> MANVNKVVRRRQVALLIALVLGIGAGGAGTWMVSEMNLKKAPPAKAPKGEPAPDMTGVVNQSFDNKVQRSAIAEAQRLNKETQTEIKKLRTEMGLVSRDLKGSQDRIRELEDQNQLLQTQLEAGKNFDSLSAEPLPGALASQGKPAPAGNVPPPTSFWPAGGGQAPAAPVMTPIQRPGMMDSQEFSLPDTGPKKPRFPWISSGSFVEAIVVEGADANASVTGDKNTAPMQLRLTGKVQMPNDEEFDLTGCFVTLEAWGDVSSERAIVRSRSISCKLGDDDIDQKIAGHVSFMGKNGIKGEVVMRNGQILLYAGGAGFLDGIGKGIEKASSTTVGVGATASMSAADIGQAGLGGGVSSAAKTLSDYYIKRAEQYHPVIPIGAGNEVTLVFQDGFQLETLEEARAKAAARKKQNQPS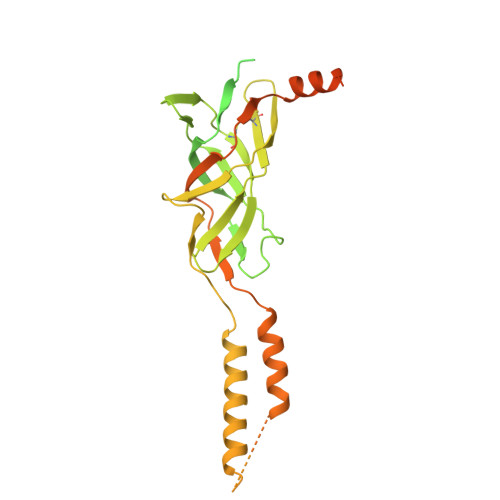ASSTPAAMPGNTPDMLKQLQDFRVGDTVDPATGQVVTQWSHPQFEK>[2x]FTEQPIDLVPNQPYPNASFDNF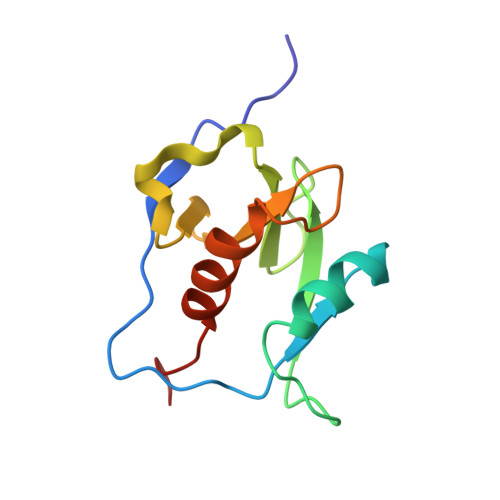KFVCDNIKFADDLNQLTGYKKPASRELKVTFFPDLNGDVVAIDYKHYTPSFKKGAKLLHKPIVWHVNNATNKATYKPNTWCIRCLWSTKPVET> METILEQQRRYHEEKERLMDVMAKEMLTKKSTLRDQINSDHRTRAMQDRYMEVSGNL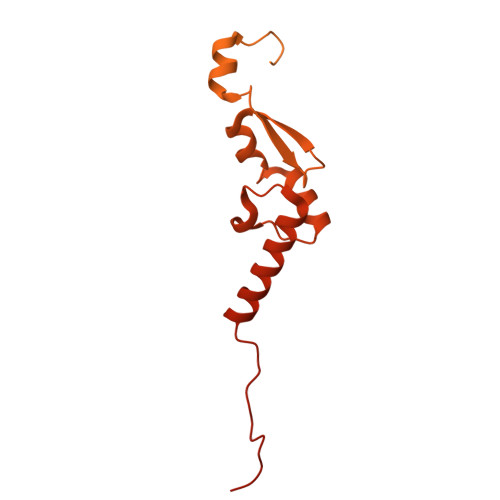RDLYDDKDGLRKEELNAISGPNEFAEFYNRLKQIKEFHRKHPNEICVPMSVEFEELLKARENPSEEAQNLVEFTDEEGYGRYLDLHDCYLKYINLKASEKLDYITYLSIFDQLFDIPKERKNAEYKRYLEMLLEYLQDYTDRVKPLQDQNELFGKIQAEFEKKWENGTFPGWPKETSSALTHAGAHLDLSAFSSWEELASLGLDRLKSALLALGLKCGGTLEERAQRLFSTKGKSLESLDTSLFAKNPKSKGTKRDTERNKDIAFLEAQIYEYVEILGEQRHLTHENVQRKQARTGEEREEEEEEQISESESEDEENEIIYNPKNLPLGWDGKPIPYWLYKLHGLNINYNCEICGNYTYRGPKAFQRHFAEWRHAHGMRCLGIPNTAHFANVTQIEDAVSLWAKLKLQKASERWQPDTEEEYEDSSGNVVNKKTYEDLKRQGLL(E)-N-({3-hydroxy-2-methyl-5-[(phosphonooxy)methyl]pyridin-4-yl}methylidene)-L-phenylalanine 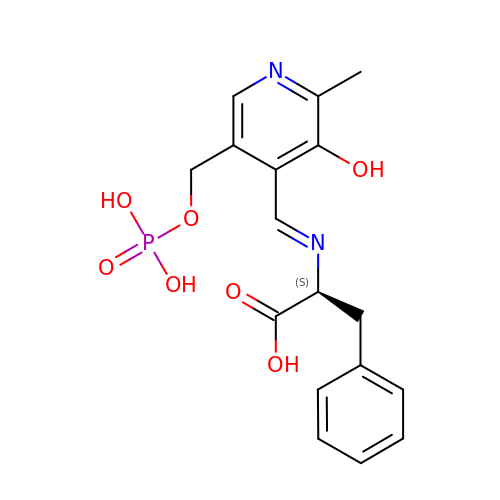| C17 H19 N2 O7 P | HMZRFMUDSWAGSO-OMPOGXFXSA-N> VLYRALVSTKWLAESIRTGKLGPGLRVLDASWYSPGTREARKEYLERHVPGASFFDIEECRDTASPYEMMLPSEAGFAEYVGRLGISNHTHVVVYDGEHLGSFYAPRVWWMFRVFGHRTVSVLNGGFRNWLKEGHPVTSEPSRPEPAVFKATLDRSLLKTYEQVLENLESKRFQLVDSRSQGRFLGTEPEPDAVGLDSGHIRGAVNMPFMDFLTEDGFEKGPEELRALFQTKKVDLSQPLIATCRKGVTACHVALAAYLCGKPDVAVYDGSWSEWFRRAPPESRV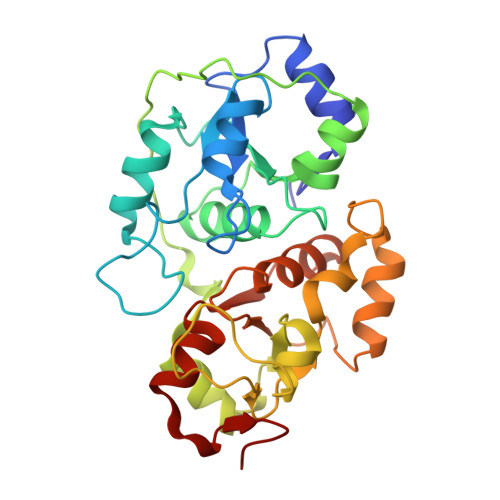SQGKS>[4x]MAKKVAVIGAGVSGLISLKCCVDEGLEPTCFERTEDIGGLWRFKENVEDGRASIYQSVITNTSKEMSCFSDFPMPEHFPNFLHNSKLLEYFRIFAKKFDLLKYIQFQTTVLSVKKCPDFSSSGQWEIVTESNGKEQSAVFDAVMVCSGHHILPHIPLQSFPGIERFKGQYFHSRQYKHPEGFEGKRILVIGIGNSASDIAVELSKKAAQVFISTRHGSWVMSRISDDGYPW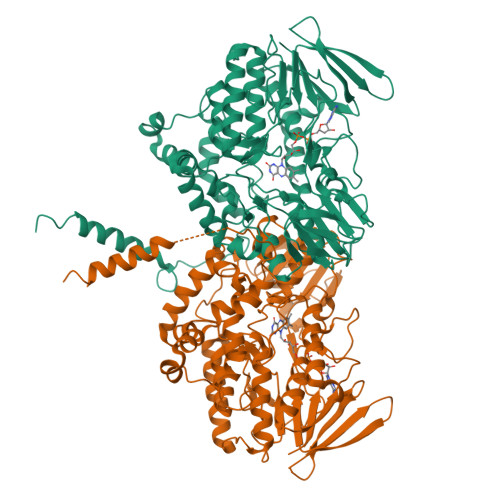DMVFHTRFSSMLRNVLPRTVVKWMMEQQMNRWFNHENYGLEPQNKYLMKEPVLNDDLPSRLLYGAIKVKSRVKELTETSAIFEDGTVEEDIDVIVFATGYTFSFPFLEDSLVKVENNMVSLYKYMFPPHLEKPTLACIGLIQPLGSIFPTVELQARWVTRVFKGLCTLPSESTMMADIIKRNEKRIDLFGESQSQILQTNYIDYLDELALEIGAKPDLLSLLLKDPKLAMKLYFGPCNSYQYRLVGPGQWEGARNAIFTQKQRILKPLKTRALKASSNFPVSFLLKILGLLAVVVAFFFQLQWF> GDPAERTWIFSGAELKQAIEGKLAPDVSDPEMRRLV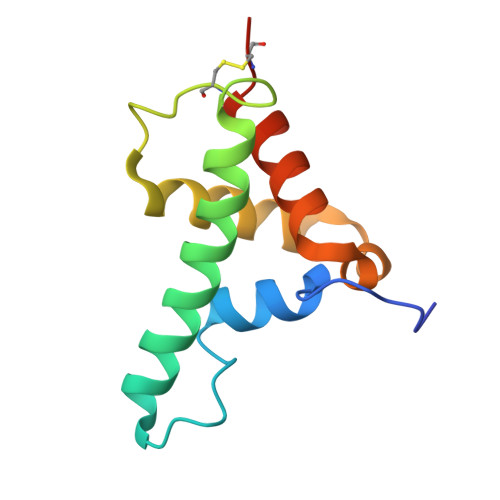SVAKSSAYIAGVADLTSGSDWCGAGAVAPHELTDRIYTYLGDMPAEKLDEQAATLVREALKVSFPCEQKSN> GSHMGSPNSPLKDSLRPKLSEEQQHIIAILLDAHHKTYDPTYADFRDFRPPVRMDGSTGSVTLDLSPLSMLPHLADLVSYSIQKVIGFAKMIPGFRDLTSDDQIVLLKSSAIEVIMLRSNQSFTMDDMSWDCGSQDYKYDVTDVSKAGHTLELIEPLIKFQVGLKKLNLHEEEHVLLMAICIVSPDRPGVQDAKLVEAIQDRLSNTLQTYIRCRHPPPGSHQLYAKMIQKLADLRSLNEEHSKQYRSLSFQP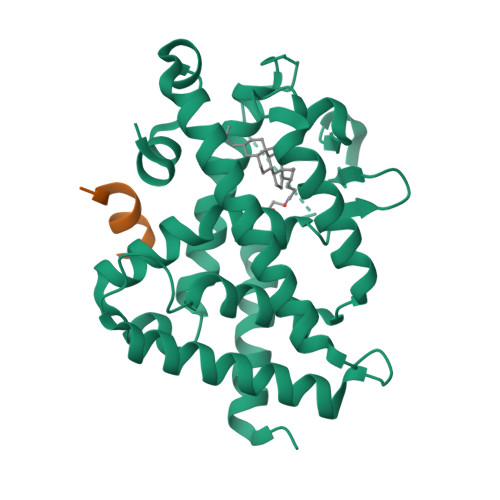ENSMKLTPLVLEVFGNEIS;> KNHPMLMNLLKDN> MLRNTDVRLFSTFALNPETSVAPHGPPRGLVNRYVSMGLPPWAAWCNKVNRYSLYRMSGVTQRSFLPKPPQEMDVIWLNERVRERVRTSRQVQNVYRQLKYPYVKTGIHYSDVLDHWVQVPMVEAAMFEVEKDGGFDNFILKRSGPELRSTYGERIRRHILVRQKEIQKNFVLQKQAQMLVESMEKEILPMEDGKKVEEV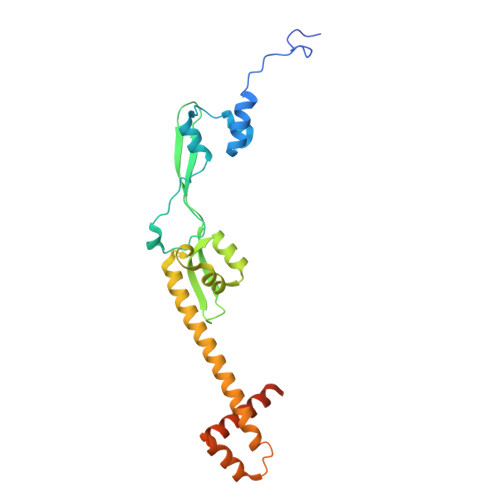LEKYGIDKEQLLRDIARAAVAKKQQLASAVPQPSHVEVSTN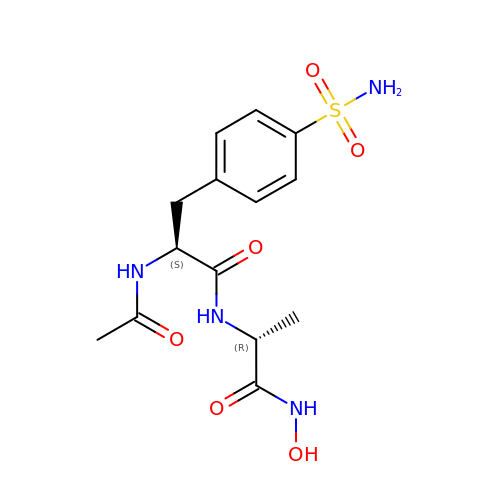(2S)-2-acetamido-N-[(2R)-1-(oxidanylamino)-1-oxidanylidene-propan-2-yl]-3-(4-sulfamoylphenyl)propanamide | C14 H20 N4 O6 S | XXSSAAVFRHGJCH-PELKAZGASA-N>MGTFIELVKNMKGYKELLLPMEMVPLPAVVLKHVKLILTSQKEHQPWMTEMALKADQCLIHKATLDLAGKATSNEAKPLIEAMQQIILAMTRELWGQIQRHHYGIVQVEHYVKQITLWQDTPQAFRGDQPKPPSFRSDGPTRGQGSFRPFFRGRGRGRGRGRGSQSPARKGPLPK[180x]

We report the capsid structure of the African cichlid nackednavirus (ACNDV), determined by cryo-EM at 3.7 Å resolution. The sequence identity with HBV is 24% and both the ACNDV capsid protein fold and the capsid architecture are very similar to those of the Hepadnaviridae and HBV in particular. The capsid is made up of 90 protein dimers to give T = 3 symmetry, with three molecules located within the asymmetric unit: chains A, B, and C. In both HBV and ACNDV, two Cp monomers associate into stable dimers via two central helices, the resulting four-helix bundles generate outward pointing spikes, and the N-termini up to the beginning of helix α3 are wrapped around the spike helices; helix α5 together with subsequent residues forms a hand-like region providing the essential inter-dimer contacts.

We used cryo-EM density maps of the pH 7.5 and 5.5 samples to build atomic-resolution structures of ACNDV capsids. At the N-terminus, the ACNDV Cp sequence starts with a small α-helix (α+), which points towards the capsid exterior surface. However, the very first residues are not visible in the cryo-EM density map. The α2-helix is wrapped around the spike helices of the partner molecule in the dimer and the spikes are made up of a four-helix bundle within the dimer helices α3 and α4 in each monomer. Comparison of the AB dimer, formed by the quasi-equivalent conformation of chains A and B, with the CC dimer, reveals that the four-helix bundles forming the spikes match well when superimposing AB with CC dimers, while the hand regions appear to be shifted. This rigid body like conformational shift between the quasi-equivalent capsid subunits observed in the cryo-EM structure agrees with the solid-state NMR measurements, which show few local conformational changes, as is further elucidated below. Secondary structure elements derived by NMR and obtained from the cryo-EM structure of ACNDV Cp at pH 7.5 agree well. Residues 66-74 were omitted in the structure because the cryo-EM map density was not well resolved at the tip of the spike for pH 7.5 and 5.5 capsids, yet the connection between the spike helices was visible in local resolution filtered maps. Unassigned cryo-EM map density located below the spikes of AB dimers but not below CC dimers was found in the ACNDV capsid maps. Likely sources of the diffuse density below AB dimers are enclosed nucleotides and/or the flexible CTD of the capsid protein.> MNKNDHPLSHLFDNNDAWVKRKLADDPQYFSRLADQQAPEYLWIGCSDSRVPANQIIGLPPGEVFVHRNIANVVVHTDLNCLSVIQFAVDLLKVKHVMVVGHYGCSGVNAALHNRRVGLADNWLHHVQDVREKHAALLEDWPLGEARYRRLIELNAIEQVVNVCRTTIVNDAWARGQPLTVHALVYGVHDGRMRNLGMAVSHAEQLDATYRRAVAALSASGAHSADNDVVAADAAQLAGAVDLIAQTIKETKHDGC

The genome of B. pseudomallei encodes for β- and γ-CAs. Our group recently reported the catalytic activity and the sulfonamide and anion inhibition profiles of the recombinant β- and γ-CAs from B. pseudomallei, named BpsβCA and BpsγCA, respectively. Besides, the bacterial CAs play a pivotal role in the life cycle and pathogenicity of the microorganism, balancing their endogenous equilibrium between CO2 and HCO3−. BpsβCA was revealed to be a tetrameric type II β-CA with a closed active site in which the zinc is tetrahedrally coordinated to Cys46, Asp48, His102, and Cys105.

Therefore, it was hypothesized that the closed conformation (called T state) observed in the structures of type II β-CAs is an allosteric form of the enzyme and, is the inactive form at pH values below 8.0. However, at pH values larger than 8.3, the closed active site is converted to an open one, with an incoming water molecule replacing the carboxylate moiety of the Asp residue, thus generating the nucleophile required in the catalytic cycle. Finally, to gain information on the open conformation of the enzyme active site, we solved the structure of the enzyme from one crystal obtained in the same crystallization condition, except pH was increased to 8.5, a value at which the enzyme was shown to possess catalytic activity. Although the structure was determined at quite a low resolution (maximum resolution 2.7 Å), we could observe that in the active site, the Asp48 is in the same position as in the structure at pH 7.5, interacting directly with the zinc ion. Nevertheless, the active form was never observed in a β-CA structure, regardless of the crystallization pH, except for in two mutants of H. influenzae CAs and a thiocyanate inhibitor complex of M. tuberculosis CA. The X-ray crystal structure of the enzyme was solved at 2.7 Å resolution and two different pH levels (7.5 and 8.5). The X-ray structure solved at two pH levels (7.5 and 8.5) showed the same “close” conformation at the active site.> MELIRIAMKKDLENDNSLMNKWATVAGLKNPNPLYDFLNHDGKTFNEFSSIVNIVKSQYPDREYELMKDYCLNLDVKTKAARSALEYADANMFFEIEDVLIDSMISCSNMKSKEYGKVYKIHRELSNSVITEFEAVKRLGKLNIKTPEMNSFSRLLLLYHYLSTGNFSPMAQLIKQIDLSE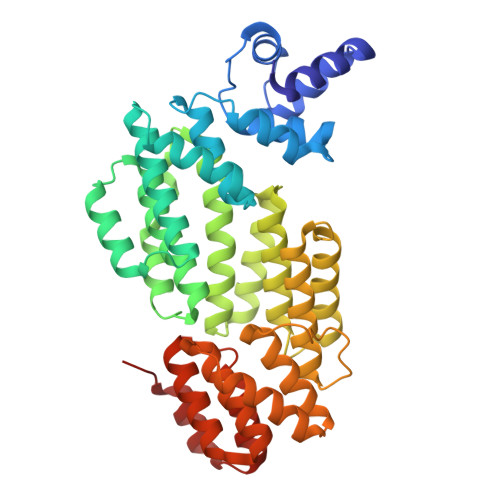ISENMYIRNTYQTRVHVLMSNIKLNENSLEECREYSKKALESTNILRFQVFSYLTIGNSLLFSNYELAQENFLKGLSISVQNENYNMIFQQALCFLNNVWRKENKWINFESDSIMDLQEQAHCFINFNENSKAKEVLDKLDLLVHNDNELAMHYYLKGRLEQNKACFYSSIEYFKKSNDKFLIRLPLLELQKMGENQKLLELLLLLEYA> MAKDIEISASESKFILEALRQNYRLDGRSFDQFRDVEITFGKEFGDVSVKMGNTKVHCRISCQIAQPYEDRPFEGLFVISTEISPMAGSQFENGNITGEDEVLCSRIIEKSVRRSGALDVEGLCIVAGSKCWAVRADVHFLDCDGGFIDASCIAVMAGLMHFKKPDITVHGEQIIVHPVNEREPVPLGILHIPICVTFSFFNPQDTEENIKGETNSEISIIDATLKEELLRDGVLTVTLNKNREVVQVSKAGGLPMDALTLMKCCHEAYSIIEKITDQILQLLKEDSEKRNKYAAMLTSENAREI;> GPDHMSRLEIYSPEGLRLDGRRWNELRRFESSINTHPHAADGSSYMEQGNNKIITLVKGPKEPRLKSQMDTSKALLNVSVNITKFSKFERSKSSHKNERRVLEIQTSLVRMFEKNVMLNIYPRTVIDIEIHVLEQDGGIMGSLINGITLALIDAGISMFDYISGISVGLYDTTPLLDTNSLEENAMSTVTLGVVGKSEKLSLLLVEDKIPLDRLENVLAIGIAGAHRVRDLMDEELRKHAQKRVSNASAR;> MAESTTLETIEIHPITFPPEVLARISPELSLQRHLSLGIRPCLRKYEEFRDVAIENNTLSRYADAGNIDTKNNILGSNVLKSGKTIVITSITGGIIEETSAAIKDLDDFGEEELFEVTKEEDIIANYASVYPVVEVERGRVGACTDEEMTISQKLHDSILHSRILPKKALKVKAGVRSANEDGTFSVLYPDELEDDTLNETNLKMKRKWSYVLYAKIVVLSRTGPVFDLCWNSLMYALQSVKLPRAFIDERASDLRMTIRTRGRSATIRETYEIICDQTKSVPLMINAKNIAFASNYGIVELDPECQLQNSDNSEEEEVDIDMDKLNTVLIADLDTEAEETSIHSTISILAAPSGNYKQLTLVGGGAKITPEMIKRSLLLSRVRADDLSTRFNI;> GSMSVQAEIGILDHVDGSSEFVSQDTKVICSVTGPIEPKARQELPTQLALEIIVRPAKGVATTREKVLEDKLRAVLTPLITRHCYPRQLCQITCQILESGEDEAEFSLRELSCCINAAFLALVDAGIALNSMCASIPIAIIKDTSDIIVDPTAEQLKISLSVHTLALEFVNGGKVVKNVLLLDSNGDFNEDQLFSLLELGEQKCQELVTNIRRIIQDNISPRLVV;> GDPHMSLSVAEKSYLYDSLASTPSIRPDGRLPHQFRPIEIFTDFLPSSNGSSRIIASDGSECIVSIKSKVVDHHVENELLQVDVDIAGQRDDALVVETITSLLNKVLKSGSGVDSSKLQLTKKYSFKIFVDVLVISSHSHPVSLISFAIYSALNSTYLPKLISAFDDLEVEELPTFHDYDMVKLDINPPLVFILAVVGNNMLLDPAANESEVANNGLIISWSNGKITSPIRSVALNDSNVKSFKPHLLKQGLAMVEKYAPDVVRSLENL;> MNVQDRRRLLGPAAAKPMAFSNTTTHVPEKKSTDLTPKGNESEQELSLHTGFIENCNGSALVEARSLGHQTSLITAVYGPRSIRGSFTSQGTISIQLKNGLLEKYNTNELKEVSSFLMGIFNSVVNLSRYPKSGIDIFVYLTYDKDLTNNPQDDDSQSKMMSSQISSLIPHCITSITLALADAGIELVDMAGAGEANGTVVSFIKNGEEIVGFWKDDGDDEDLLECLDRCKEQYNRYRDLMI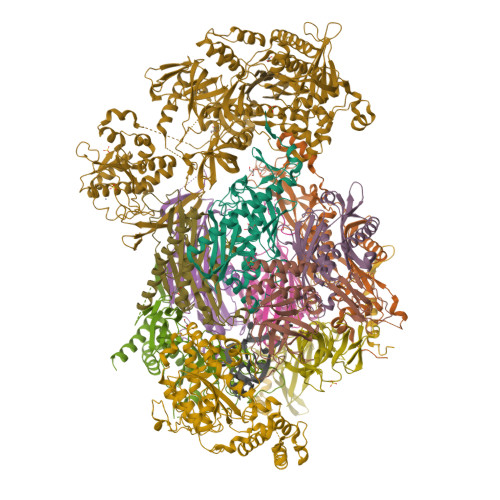SCLMNQET;> GDPHMSTFIFPGDSFPVDPTTPVKLGPGIYCDPNTQEIRPVNTGVLHVSAKGKSGVQTAYIDYSSKRYIPSVNDFVIGVIIGTFSDSYKVSLQNFSSSVSLSYMAFPNASKKNRPTLQVGDLVYARVCTAEKELEAEIECFDSTTGRDAGFGILEDGMIIDVNLNFARQLLFNNDFPLLKVLAAHTKFEVAIGLNGKIWVKCEELSNTLACYRTIMECCQKNDTAAFKDIAKRQFKEILTVKEE;> GDPHMSEVITITKRNGAFQNSSNLSYNNTGISDDENDEEDIYMHDVNSASKSESDSQIVTPGELVTDDPIWMRGHGTYFLDNMTYSSVAGTVSRVNRLLSVIPLKGRYAPETGDHVVGRIAEVGNKRWKVDIGGKQHAVLMLGSVNLPGGILRRKSESDELQMRSFLKEGDLLNAEVQSLFQDGSASLHTRSLKYGKLRNGMFCQVPSSLIVRAKNHTHNLPGNITVVLGVNGYIWLRKTSQMDLARDTPSANNSSSIKSTGPTGAVSLNPSITRLEEESSWQIYSDENDPSISNNIRQAICRYANVIKALAFCEIGITQQRIVSAYEASMVYSNVGELIEKNVMESIGSDILTAEKMRGNGN;> GDPHMACNFQFPEIAYPGKLICPQYGTENKDGEDIIFNYVPGPGTKLIQYEHNGRTLEAITATLVGTVRCEEEKKTDQEEEREGTDQSTEEEKSVDASPNDVTRRTVKNILVSVLPGTEKGRKTNKYANNDFANNLPKEGDIVLTRVTRLSLQRANVEILAVEDKPSPIDSGIGSNGSGIVAAGGGSGAATFSVSQASSDLGETFRGIIRSQDVRSTDRDRVKVIECFKPGDIVRAQVLSLGDGTNYYLTTARNDLGVVFARAANGAGGLMYATDWQMMTSPVTGATEKRKCAKPF;> SLMVEKPQLKFKSPIDNSESHPFIPLLKEKPNALKPLSESLRLVDDDENNPSHYPHPYEYEIDHQEYSPEILQIREEIPSKSWDDSVPIWVDTSTELESMLEDLKNTKEIAVNLEHHDYRSYYGIVCLMQISTRERDYLVDTLKLRENLHILNEVFTNPSIVKVFHGAFMDIIWLQRDLGLYVVGLFDTYHASKAIGLPRHSLAYLLENFANFKTSKKYQLADWRIRPLSKPMTAYARADTHFLLNIYDQLRNKLIESNKLAGVLYESRNVAKRRFEYSKYRPLTPSSEVYSPIEKESPWKILMYQYNIPPEREVLVRELYQWRDLIARRDDESPRFVMPNQLLAALVAYTPTDVIGVVSLTNGVTEHVRQNAKLLANLIRDALRNIKNTNEEATPIPSSETKADGILLETISVPQIRDVMERFSVLCNSNISKSRAKPVTNSSILLGKILPREEHDIAYSKDGLPNKVKTEDIRIRAQNFKSALANLEDIIFEIEKPLVVPVKLEEIKTVDPASAPNHSPEIDNLDDLVVLKKKNIQKKQPAKEKGVTEKDAVDYSKI;> SLMSVPAIAPRRKRLADGLSVTQKVFVRSRNGGATKIVREHYLRSDIPCLSRSCTKCPQIVVPDAQNELPKFILSDSPLELSAPIGKHYVVLDTNVVLQAIDLLENPNCFFDVIVPQIVLDEVRNKSYPVYTRLRTLCRDSDDHKRFIVFHNEFSEHTFVERLPNETINDRNNRAIRKTCQWYSEHLKPYDINVVLVTNDRLNREAATKEVESNIITKSLVQYIELLPNADDIRDSIPQMDSFDKDLERDTFSDFTFPEYYSTARVMGGLKNGVLYQGNIQISEYNFLEGSVSLPRFSKPVLIVGQKNLNRAFNGDQVIVELLPQSEWKAPSSIVLDSEHFDVNDNPDIEAGDDDDNNESSSNTTVISDKQRRLLAKDAMIAQRSKKIQPTAKVVYIQRRSWRQYVGQLAPSSVDPQSSSTQNVFVILMDKCLPKVRIRTRRAAELLDKRIVISIDSWPTTHKYPLGHFVRDLGTIESAQAETEALLLEHDVEYRPFSKKVLECLPAEGHDWKAPTKLDDPEAVSKDPLLTKRKDLRDKLICSIDPPGCVDINDALHAKKLPNGNWEVGVHIADVTHFVKPGTALDAEGAARGTSVYLVDKRIDMLPMLLGTDLCSLKPYVDRFAFSVIWELDDSANIVNVNFMKSVIRSREAFSYEQAQLRIDDKTQNDELTMGMRALLKLSVKLKQKRLEAGALNLASPEVKVHMDSETSDPNEVEIKKLLATNSLVEEFMLLANISVARKIYDAFPQTAMLRRHAAPPSTNFEILNEMLNTRKNMSISLESSKALADSLDRCVDPEDPYFNTLVRIMSTRCMMAAQYFYSGAYSYPDFRHYGLAVDIYTHFTSPIRRYCDVVAHRQLAGAIGYEPLSLTHRDKNKMDMICRNINRKHRNAQFAGRASIEYYVGQVMRNNESTETGYVIKVFNNGIVVLVPKFGVEGLIRLDNLTEDPNSAAFDEVEYKLTFVPTNSDKPRDVYVFDKVEVQVRSVMDPITSKRKAELLLK>[4x]MKEFYLTVEQIGDSIFERYIDSNGRERTREVEYKPSLFAHCPESQATKYFDIYGKPCTRKLFANMRDASQWIKRMEDIGLEALGMDDFKLAYLSDTYNYEIKYDHTKIRVANFDIEVTSPDGFPEPSQAKHPIDAITHYDSIDDRFYVFDLLNSPYGNVEEWSIEIAAKLQEQGGDEVPSEIIDKIIYMPFDNEKELLMEYLNFWQQKTPVILTGWNVESFAIPYVYNRIKNIFGESTAKRLSPHRKTRVKVIENMYGSREIITLFGISVLDYIDLYKKFSFTNQPSYSLDYISEFELNVGKLKYDGPISKLRESNHQRYISYNIIAVY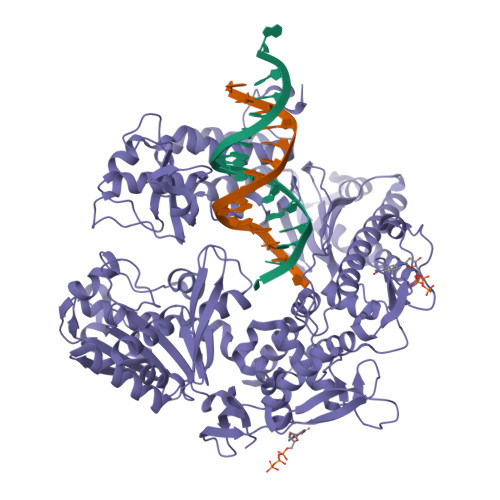RVLQIDAKRQFINLSLDMGYYAKIQIQSVFSPIKTWDAIIFNSLKEQNKVIPQGRSHPVQPYPGAFVKEPIPNRYKYVMSFDLTSLYPSIIRQVNISPETIAGTFKVAPLHDYINAVAERPSDVYSCSPNGMMYYKDRDGVVPTEITKVFNQRKEHKGYMLAAQRNGEIIKEALHNPNLSVDEPLDVDYRFDFSDEIKEKIKKLSAKSLNEMLFRAQRTEVAGMTAQINRKLLINSLYGALGNVWFRYYDLRNATAITTFGQMALQWIERKVNEYLNEVCGTEGEAFVLYGDTDSIYVSADKIIDKVGESKFRDTNHWVDFLDKFARERMEPAIDRGFREMCEYMNNKQHLMFMDREAIAGPPLGSKGIGGFWTGKKRYALNVWDMEGTRYAEPKLKIMGLETQKSSTPKAVQKALKECIRRMLQEGEESLQEYFKEFEKEFRQLNYISIASVSSANNIAKYDVGGFPGPKCPFHIRGILTYNRAIKGNIDAPQVVEGEKVYVLPLREGNPFGDKCIAWPSGTEITDLIKDDVLHWMDYTVLLEKTFIKPLEGFTSAAKLDYEKKASLFDMFDF(R)-N-(3-(1H-indol-3-yl)-1-oxo-1-(pyridin-4-ylamino)propan-2-yl)-4-(4-(4-chlorophenyl)piperazin-1-yl)-2-fluorobenzamide | C33 H30 Cl F 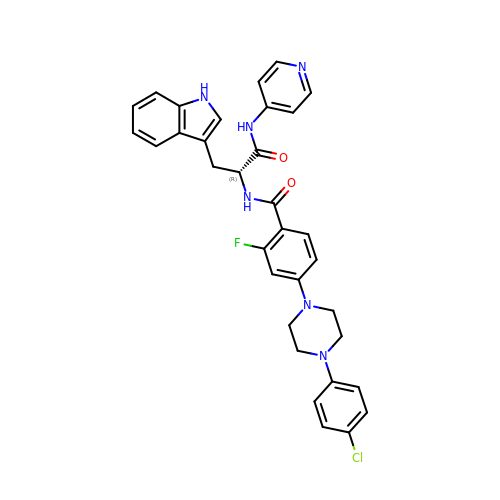N6 O2 | JVZAEFLHUYIXPY-WJOKGBTCSA-N> AQDDSTPDSLFAGLVGEYYGTNSQLNNISDFRALVDSKEADATFEAANISYGRGSSDVAKGTHLQEFLGSDASTLSTDPGDNTDGGIYLQGYVYLEAGTYNFKVTADDGYEITINGNPVATVDNNQSVYTVTHASFTISESGYQAIDMIWWDQGGDYVFQPTLSADGGSTYFVLDSAILSSTGETPYTTA

MpPA14 (Marinomonas primoryensis PA14 domain) lectin is a domain of a 1.5-MDa adhesin responsible for a symbiotic bacterium-diatom interaction in Antarctica. Bioinformatic analyses indicated the presence of an ∼20-kDa domain near the C terminus of MpIBP that is a member of the PA14 family, which is a carbohydrate-binding lectin module widely distributed across several kingdoms of life. PA14 domains share a β-sandwich fold and the presence of two consecutive aspartate residues in a cis peptide linkage (DcisD). The DcisD motif coordinates a Ca2+ ion that is directly involved in binding polar vicinal hydroxyl groups of various carbohydrates.

Mannose bound MpPA14 slightly more weakly than glucose. The electron density map for the mannose-MpPA14 complex indicated that the sugar bound in two distinct conformations. Like glucose, d-mannose bound MpPA14 via the 3,4-diol. However, since the mannose C-2 hydroxyl moiety is in an axial position, its oxygen atom may clash with the β-carbon of the Ser130, as they are only 3 Å away from each other. In addition, as the C-2 and C-3 hydroxyl groups of mannose are positioned in cis, they may form an intramolecular hydrogen bond that further weakens the 3,4-diol from binding Ca1. Alternatively, β-mannopyranose can bind MpPA14 using a second configuration where its 2,3-diol anchors the saccharide ring in an inverted fashion, allowing the ring oxygen to hydrogen bond with the side chain amide group of the Gln156. However, α-mannopyranose failed to fit into the electron density via this binding mode, which indicates that MpPA14 can only recognize the less prevalent β-anomer in the equilibrium via its 2,3-diol (33% β-mannopyranose as opposed to 62% α-mannopyranose at 30°C). This apparent lack of one distinct stable binding configuration explains the relatively inferior affinity of mannose compared to glucose.> MHHHHHHSSGRENLYFQGPEL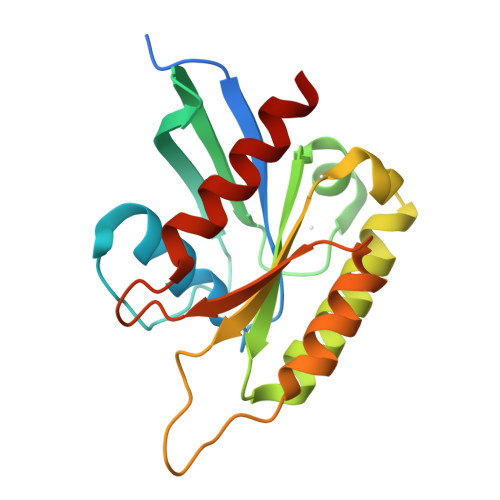KVGIVGNLSSGKSALVHRYLTGTYVQEESPEGGRFKKEIVVDGQSYLLLIRDEGGPPELQFAAWVDAVVFVFSLEDEISFQTVYNYFLRLCSFRNASEVPMVLVGTQDAISAANPRVIDDSRARKLSTDLKRCTYYETCATYGLNVERVFQDVAQKVVALRKK> MNTNNIKKYAPQARNDFRDAVIQKLTTLGIAADKKGNLQIAEAETIGETVRYGQFDYPLSTLPRRERLVKRAREQGFEVLVEHCAYTWFNRLCAIRYMELHGYLDHGFRMLSHPETPTAFEVLDHVPEVAEALLPESKAQLVEMKLSGNQDEALYRELLLGQCHALHHAMPFLFEAVDDEAELLLPDNLTRTDSILRGLVDDIPEEDWEQVEVIGWLYQFYISEKKDAVIGKVVKSEDIPAATQLFTPNWIVQYLVQNSVGRQWLQTYPDSPLKDKMEYYIEPAEQTPEVQAQLAAITPASIEPESIKVLDPACGSGHILTEAYNVLKAIYEERGYRTRDIPQLILENNIFGLDIDDRAAQLSGFAMLMLARQDDRRILGRGVRLNIVSLQESKLDIAEVWTKLNFHQHMQRGSMGDMFTQGTALANTDSAEYKLLMRTLALFTSAKTLGSLIQVPQEDEAALKAFLERLYRLAVEGDIQQKEAAAELIPYIQQAWILAQRYDAVVANPPYMGGKGMNGDLKEFAKKQFPDSKSDLFAMFMQHAFSLLKENGFNAQVNMQSWMFLSSYEALRGWLLDNKTFITMAHLGARAFGQISGEVVQTTAWVIKNNHSGFYKPVFFRLVDDNEEHKKNNLLNRMNCFKNTLQNDFKKIPGSPIAYWATLAFINSFLKLPALGTRAVKGLDTNGSIDVFLRRWPEVSINSFDALGKGNSKWFPIAKGGELRKWFGNHEYIINYENDGIELRKNKANLRNKDMYFQEGGTWTVVSTTGFSMRYMPKGFLFDQGGSAVFCENNDELSIYNILACMNSKYINYSASLICPTLNFTTGDVRKFPVIKNNHLEDLAKKAIEISKADWNQFETSWEFSKNKLIEHKGNVAYSYASYCNFQDKLYEQLVNIEKNINNIIEEILGFKIETTENSELITLNSNKIYRYGQSETNDTFLNRHRSDTISELISYSVGCQMGRYSLDREGLVYAHEGNKGFAELAAEGAYKTFPADNDGILPLMDDEWFEDDVTSRVKEFVRTVWGEEHLQENLEFIAESLCLYAIKPKKGESALETIRRYLSTQFWKDHMKMYKKRPIYWLFSSGKEKAFECLVYLHRYNDATLSRMRTEYVVPLLARYQANIDRLNDQLDEASGGEATRLKRERDSLIKKFSELRSYDDRLRHYADMRISIDLDDGVKVNYGKFGDLLADVKAITGNAPEAI

Anti-phage systems of the BREX (BacteRiophage EXclusion) superfamily rely on site-specific epigenetic DNA methylation to discriminate between the host and invading DNA. We demonstrate that in Type I BREX systems, defense and methylation require BREX site DNA binding by the BrxX (PglX) methyltransferase employing S-adenosyl methionine as a cofactor. We show that BrxX contains MTD and TRD homologous to those of Type IIL R-M enzymes, and, in addition, contains NTD, CTD, and insertion loop in the MTD specific to BrxX proteins. We show that BrxX alone does not methylate DNA, and BREX activity requires an assembly of a supramolecular BrxBCXZ immune complex.

A 2.2 Å cryogenic electron microscopy (cryoEM) structure of a BrxX-DNA complex shows that both target recognition and methyltransferase domains (MTDs) are involved in sequence-specific recognition of BREX sites. However, when BrxX was incubated with a 43 bp dsDNA fragment containing two BREX sites in a head-to-tail (H2T) arrangement (DNA H2T) in the presence of SAM, a DNA-bound complex accounted for the majority of 2D class averages. Single-particle analysis of 11,152 movie dataset demonstrated the formation of a 1:1 complex (BrxX:DNA) that was highly homogenous despite the presence of two BREX sites. Only the first (from the 5′-end) binding site was occupied, suggesting that a stretch of DNA downstream of a BREX site is essential for BrxX binding. The DNA-bound BrxX is a bi-lobed Pacman-like monomer consisting of four domains. The DNA bound to BrxX is bent by ~33°, with the most prominent distortion occurring around the six-base pair recognition sequence embedded between the MTD and TRD. The fifth adenine of the GGTAAG sequence is rotated out of the DNA backbone together with its deoxyribose moiety and the neighboring phosphodiester groups and is nestled in the active site of the MTD. The TRD contributes to the recognition of the first four base pairs of the recognition sequence. Our analysis identified a critical loop (residues 587–601) in E. coli BrxX MTD that confers specificity to the recognition of the final base pair of the BREX site. The superposition of the two structures makes it clear that it is the “upper jaw” of the BrxX monomer that closes around the DNA upon recognition as the MTD moves 19.7° between the open and closed states (left).>[7x]SLPSFIEHSSFGVKESNPYNKLFEERIIFLGVQVDDASANDIMAQLLVLESLDPDRDITMYINSPGGGFTSLMAIYDTMQYVRADIQTVCLGQAASAAAVLLAAGTPGKRMALPNARVLIHQPSLSGVIQGQFSDLEIQAAEIERMRTLMETTLARHTGKDAGVIRKDTDRDKILTAEEAKDYGIIDTVLEYRKLSAQ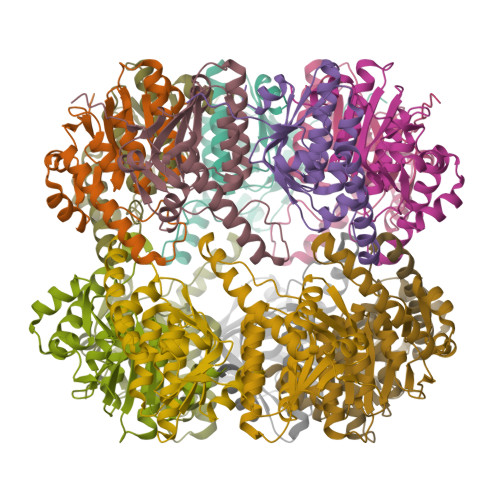TA;>[7x]MRSNSQGLSLTDSVYERLLSERIIFLGSEVNDEIANRLCAQILLLAAEDASKDISLYINSPGGSISAGMAIYDTMVLAPCDIATYAMGMAASMGEFLLAAGTKGKRYALPHARILMHQPLGGVTGSAADIAIQAEQFAVIKKEMFRLNAEFTGQPIERIEADSDRDRWFTAAEALEYGFVDHIITRAHVNGEAQ>[2x]VEDEEHIDLPPGFRFHPTDEELITHYLKPKVFNTFFSATAIGEVDLNKIEPWDLPWKAKMGEKEWYFFCVRDRKYPTGLRTNRATEAGYWKATGKDKEIFKG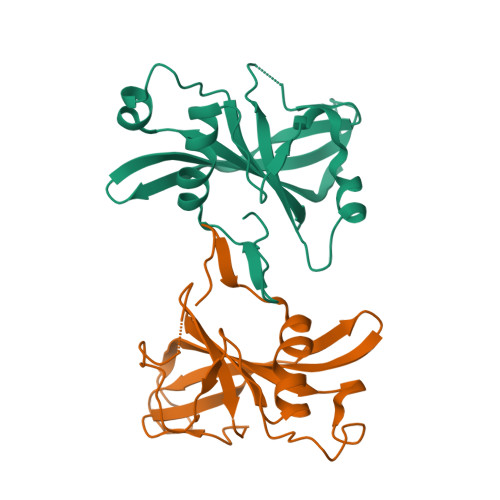KSLVGMKKTLVFYKGRAPKGVKTNWVMHEYRLEGKYCIENLPQTAKNEWVICRVFQK6-{[(2,5-dichlorophenyl)amino]methyl}pyrido[2,3-d]pyrimidine-2,4-diamine 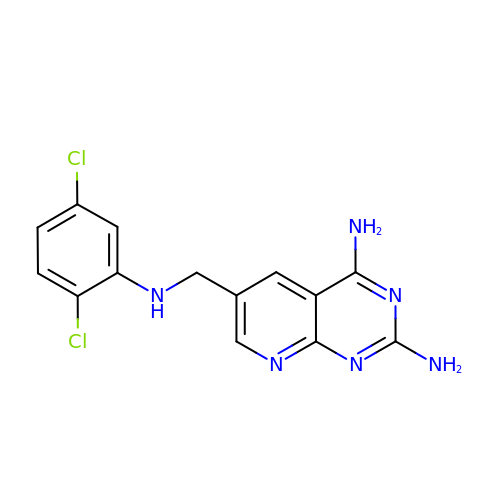| C14 H12 Cl2 N6 | RSPDQFOJWPXTPN-UHFFFAOYSA-N> RGSHGGSMGPQVVKVEDIDFATKFTPPTGSTELDLIGYGNTGMEIETVEIRFTAIGFYAEPSISEHLQKWKGTPSSNLVEDDSGFHKELIQAPVEKAVRISIIKGIKGLPYGSALQSSLRDRLVNNDLFEEEEEEALEKLAEFFQPHNLPKGTNIIYHWATPSSVKVSLSEEGKMPEDVAYTIDDAHVAEALLDLYLGENTITPSTLASVAEAIAA

Chalcone isomerase–like (CHIL) protein is a noncatalytic protein that enhances flavonoid content in green plants by serving as a metabolite binder and a rectifier of chalcone synthase (CHS). Rectification of CHS catalysis occurs through direct protein–protein interactions between CHIL and CHS, which alter CHS kinetics and product profiles, favoring naringenin chalcone (NC) production. The chalcone isomerase–like (CHIL) protein family is noncatalytic, yet it shares a “CHI fold” with CHI. The protein X-ray crystal structures of PpCHIL-A and VvCHIL reveal CHI-type α/β folds with high structural homology to each other.

Two CHILs are studied that represent distantly related species in the lineage of green plants: the lone CHIL from grape seed, Vitis vinifera (VvCHIL), and one of two known CHILs from the bryophyte, Physcomitrella patens (PpCHIL-A). PpCHIL-A and MtCHI-I have a high degree of structural similarity and align well to each other (C⍺-based RMS = 1.213 Å). This structural superposition reveals that PpCHIL-A contains a potential ligand-binding pocket that is analogous in some ways to the active site of MtCHI-I and complementary to the shape of naringenin, as it is oriented in the structure of MtCHI-I. Within the putative ligand-binding pocket, the tryptophan (W221 by VvCHIL numbering) is highly conserved across green plants with the notable exceptions of the two CHILs from P. patens, both of which possess a leucine in the same position (L188 by PpCHIL-A numbering). In summary, the structures of VvCHIL and PpCHIL-A suggest that PpCHIL-A may possess a binding pocket that is suitable to accommodate naringenin. This structural hypothesis is consistent with the observation that naringenin binding to PpCHIL-A has a stabilizing effect, which is similar to MsCHI-II. Supporting this idea, analysis of the VvCHIL-binding pocket reveals a pocket volume of 20.8 A3, whereas the volume of the PpCHIL-A–binding pocket is significantly larger, calculated to be 50.7 A3. The X-ray crystal structures of PpCHIL-A and VvCHIL were not available through the Protein Data Bank (PDB) prior to release of the AlphaFold predictions, and indeed, the PpCHIL-A X-ray crystal structure shows significant positional deviations when compared with the AlphaFold-predicted structure. A significant error in the AlphaFold model occurs in the β-hairpin motif abutting the ligand-binding site, which has significance in understanding protein–ligand interactions. The protein X-ray crystal structure of PpCHIL-A reveals a binding pocket that is analogous in some ways to the active site of MtCHI-I, and molecular dynamics simulations have revealed that the active-site architecture of MtCHI-I directs stereoselective ring closure of NC to form 2S-naringenin instead of 2R-naringenin.> XAMVSAFLKQA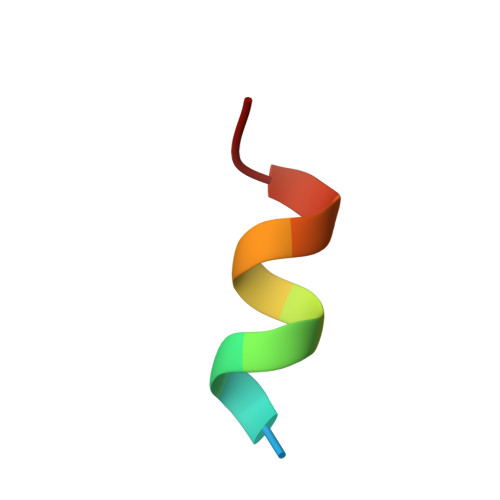W>[3x]MTIKVGINGFGRIGRIVFRAAQKRSDIEIVAINDLLDADYMAYMLKYDSTHGRFDGTVEVKDGHLIVNGKKIRVTAERDPANLKWDEVGVDVVAEATGLFLTDETARKHITAGAKKVVMTGPSKDNTPMFVKGANFDKYAGQDIVSNASCTTNCLAPLAKVINDNFGIIEGLMTTVHATTATQKTVDGPSHKDWRGGRGASQNIIPSSTGAAKAVGKVLPELNGKLTGMAFRVPTPNVSVVDLTVRLEKAATYEQIKAAVKAAAEGEMKGVLGYTEDDVVSTDFNGEVCTSVFDAKAGIALNDNFVKLVSWYDNETGYSNKVLDLIAHISK;> MVKVGINGFGRIGRLVLRVCMEKGVRVVAVNDPFIDPEYMVYMFKYDSTHGRYKGTVEHKNGRLVVDNLEINVFQCKEPKEIPWSSVGNPYVVEATGVYLSIEAASGHISSGARRVIVTAPSPDAPMLVMGVNEKDYNPGSMTVVSNASCTTNCLAPLA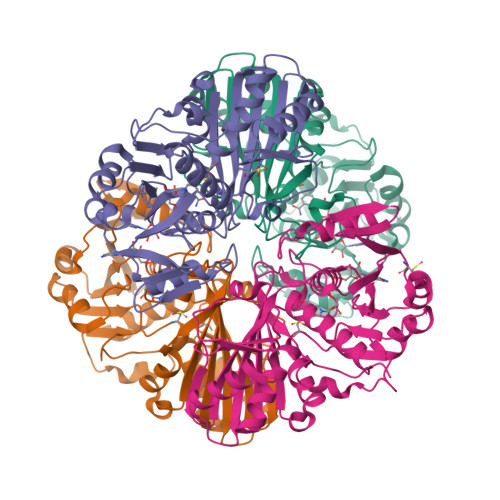KVIHERFGIVEGLMTTVHAYTATQKTVDGPSKKDWRGGRGAHQNIIPSSTGAAKAVGKVIPELNGKLTGMAFRVPTPNVSVVDLTCRLAQPASYTAIKEAVKAAAKGPMAGILAYTEDQVVSTDFNGDSHSSIFDAKAGIALNDNFVKLVSWYDNEYGYSHRVVDLLRYMFSREK> MKESYYSIGEVSKLANVSIKALRYYDKIDLFKPAYVDPDTSYRYYTDSQLIHLDLIKSLKYIGTPLEEMKKAQDLEMEELFAFYTEQERQIREKLDFLS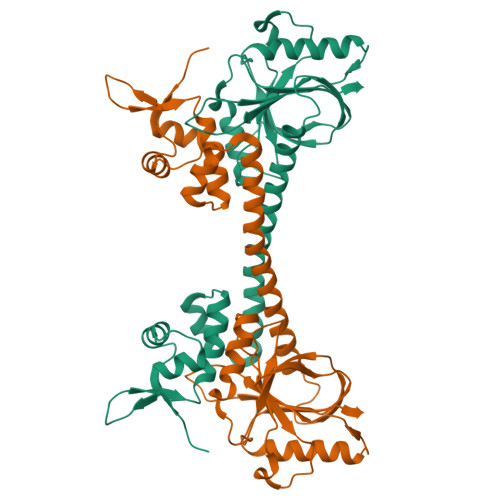ALEQTISLVKKRMKRQMEYPALGEVFVLDEEEIRIIQTEAEGIGPENVLNASYSKLKKFIESADGFTNNSYGATFSFQPYTSIDEMTYRHIFTPVLTNKQISSITPDMEITTIPKGRYACIAYNFSPEHYFLNLQKLIKYIADRQLTVVSDVYQLIIPIHYSPKKQEEYRVEMKIEIAE>[2x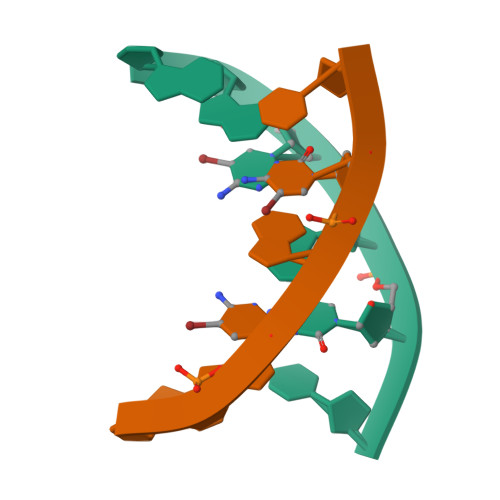]GGCGCC>MLGILNKMFDPTKRTLNRYEKIANDIDAIRGDYENLSDDALKHKTIEFKERLEKGATTDDLLVEAFAVVREASRRVTGMFPFKVQLMGGVALHDGNIAEMKTGEGKTLTSTLPVYLNALTGKGVHVVTVNEYLASRDAEQMGKIFEFLGLTVGLNLNSMSKDEKREAYAADITYSTNNELGFDYLRDNMVLYKEQMVQRPLHFAVIDEVDSILIDEARTPLIISGQAAKSTKLYVQANAFVRTLKAEKDYTYDIKTKAVQLTEEGMTKAEKAFGIDNLFDVKHVALNHHINQALKAHVAMQKDVDYVVEDGQVVIVDSFTGRLMKGRRYSEGLHQAIEAKEGLEIQNESMTLATITFQNYFRMYEKLAGMTGTAKTEEEEFRNIYNMQVVTIPTNRPVVRDDRPDLIYRTMEGKFKAVAEDVAQRYMTGQPVLVGTVAVETSELISKLLKNKGIPHQVLNAKNHEREAQIIEEAGQKGAVTIATNMAGRGTDIKLGEGVKELGGLAVVGTERHESRRIDNQLRGRSGRQGDPGITQFYLSMEDELMRRFGAERTMAMLDRFGMDDSTPIQSKMVSRAVESSQKRVEGNNFDSRKQLLQYDDVLRQQREVIYKQRFEVIDSENLREIVENMIKSSLERAIAAYTPREELPEEWKLDGLVDLINTTYLDEGALEKSDIFGKEPDEMLELIMDRIITKYNEKEEQFGKEQMREFEKVIVLRAVDSKWMDHIDAMDQLRQGIHLRAYAQTNPLREYQMEGFAMFEHMIESIEDEVA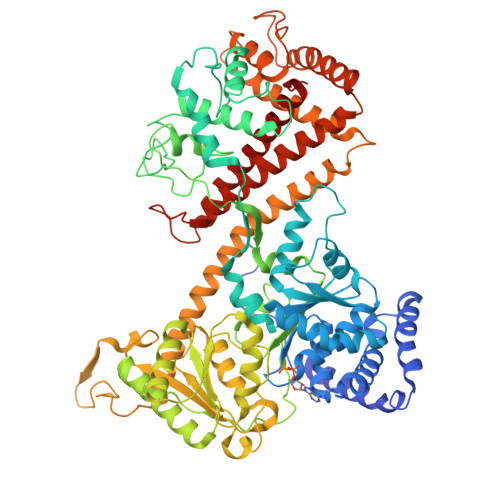KFVMKAEI[2x]>[2x]SMRTAQEVETYRRSKEITVRGHNCPKPVLNFYEANFPANVMDVIARQNFTEPTAIQAQGWPVALSGLDMVGVAQTGSGKTLS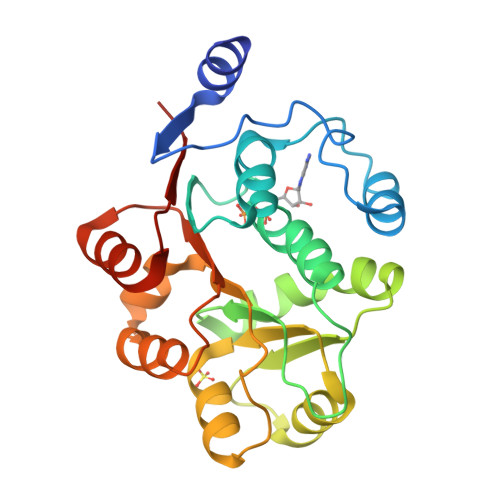YLLPAIVHINHQPFLERGDGPICLVLAPTRELAQQVQQVAAEYCRACRLKSTCIYGGAPKGPQIRDLERGVEICIATPGRLIDFLECGKTNLRRTTYLVLDEADRMLDMGFEPQIRKIVDQIRPDRQTLMWSATWPKEVRQLAEDFLKDYIHINIGALEL> MNFSSSARWLAVRQSQTLGHTTRATVAAGRRVLAHSPAATEFTSFQSLHIGGDVCKLPLAVALGAAPSALGYGSAKHNQQRQYATLGSGWSFSKVQYTKYRITKPWTTDTTFDDIILSQPSKEDFAKFTKEAPLFLRFLKLVTDVEGRQEAFIQFAKRCENGLTVEKDVYVTKKELVDCLWKNGYTDT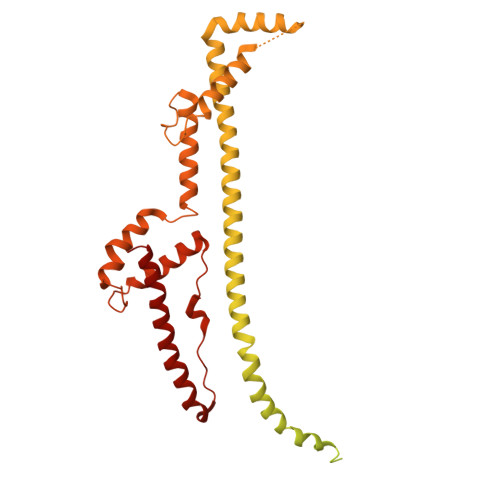EINAFEIAFPADYKFHYPELAVLFDLTEEDCYKYCIRQRAATPEELVELKYTKPKNLVSSYGLCFLGVWFGLSNTVLSNAWFYSKTFPFGAVFYMLGSYFYRDIREKLWKEEKSLIHTAQENKNMGEESVYKQMKKYATDTKCLDYLSTFRTEVEDQIANYKVALVSQMRRQLTERLVEKLNGIQQAEKLIQGSLQDVMIREIVSSFKDLYKSRPELHDAAMQSAIQGLSGSDGAMDPVGAHFKASLQELAKVNLSTATADPMGTVVQRVAAVFQKREKEFLDTFTVKATEAQEIKTIVDKCHKGNTFDFHALSDEELRRLEQLYSTVNNRVGFETIHENSIKPVAPLSENSKGFVEFVNTQLEITKAKLRNARLTAFAHAFV>[2x]PTTCLNEGAIGYMAIDILQSQNIETITINDNEYKLNKFNNIKDYISKVWGAASVYNLDLGNDYTKWQSSLDNVETDNIKNYINGHDNVYYNPGGKNKYLIIEASKELKWKGNLNNNKFNVNLKSIFSNAENLKVGHSDLLKLFSSIV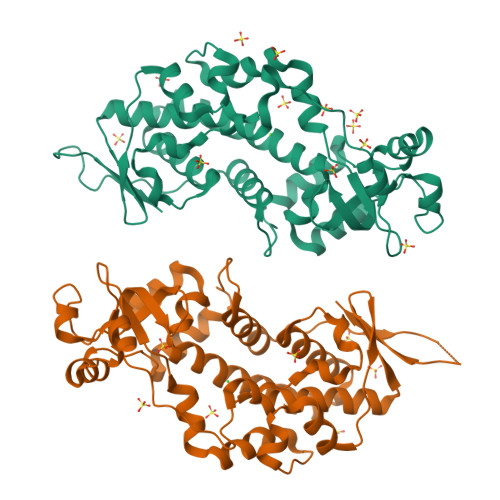NSKGSDNQKKVLNSLLDNINDRRLKKLVSTGQWTEAISDSVANEIAKNNKLTSIKAQLGSQKTQNVMIDANGHDLLKIDYDKTFVTANDLKNKIIDKNKLENAKNYFKIQNNDKILEDIKSKFSKNINENIKGSIRDHAKLIEFTENKKFNTINDNSNSDSKIKSITCKVLEHHHHHH> MKINRQQYAESYGPTVGDEV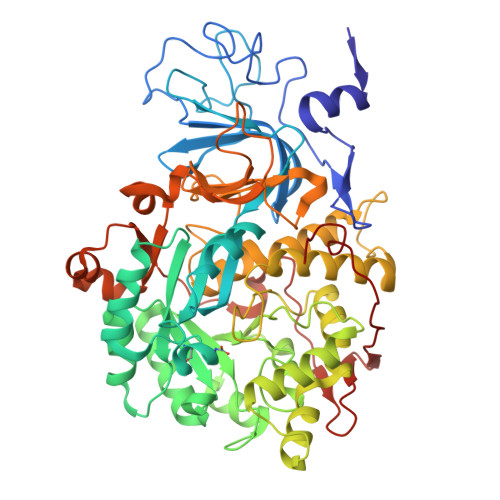RLADTDLWIEVEKDYTTYGDEVNFGGGKVLREGMGENGTYTRTENVLDLLLTNALILDYTGIYKADIGVKDGYIVGIGKGGNPDIMDGVTPNMIVGTATEVIAAEGKIVTAGGIDTHVHFINPDQVDVALANGITTLFGGGTGPAEGSKATTVTPGPWNIEKMLKSTEGLPINVGILGKGHGSSIAPIMEQIDAGAAGLKIHEDWGATPASIDRSLTVADEADVQVAIHSDTLNEAGFLEDTLRAINGRVIHSFHVEGAGGGHAPDIMAMAGHPNVLPSSTNPTRPFTVNTIDEHLDMLMVCHHLKQNIPEDVAFADSRIRPETIAAEDILHDLGIISMMSTDALAMGRAGEMVLRTWQTADKMKKQRGPLAEEKNGSDNFRLKRYVSKYTINPAIAQGIAHEVGSIEEGKFADLVLWEPKFFGVKADRVIKGGIIAYAQIGDPSASIPTPQPVMGRRMYGTVGDLIHDTNITFMSKSSIQQGVPAKLGLKRRIGTVKNCRNIGKKDMKWNDVTTDIDINPETYEVKVDGEVLTCEPVKELPMAQRYFLF>PPKMNPVVEPLSWMLGTWLSDPPGAGTYPTLQPFQYLEEVHISHVGQPMLNF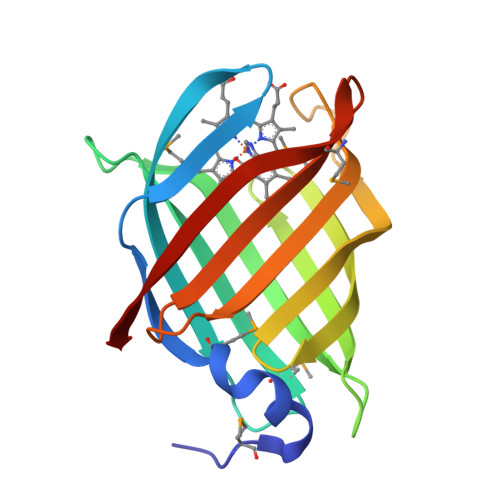SFNSFHPDTRKPMHRECGFIRLKPDTNKVAFVSAQNTGVVEVEEGEVNGQELCIASHSIARISFAKEPHVEQITRKFRLNSEGKLEQTVSMATTTQPMTQHLHVTYKKVTP[2x]> AMEVHPISEFASPFEVFKCIERDFKVAGLLESIGGPQYKARYSVIAWSTNGYLKIHDDPVNILNGYLKDLKLADIPGLFKGGMIGYISYDAVRFWEKIRDLKPAAEDWPYAEFFTPDNIIIYDHNEGKVYVNADLSSVGGCGDIGEFKVSFYDESLNKNSYERIVSESLEYIRSGYIFQVVLSRFYRYIFSGDPLRIYYNLRRINPSPYMFYLKFDEKYLIGSSPELLFRVQDNIVETYPIAGTRPRGADQEEDLKLELELMNSEKDKAEHLMLVDLARNDLGKVCVPGTVKVPELMYVEKYSHVQHIVSKVIGTLKKKYNALNVLSATFPA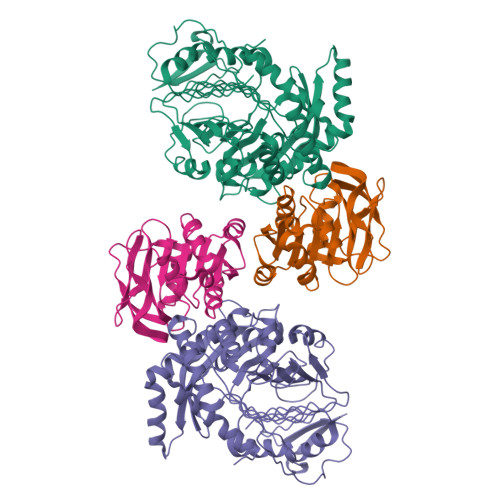GTVSGAPKPMAMNIIETLEEYKRGPYAGAVGFISADGNAEFAIAIRTAFLNKELLRIHAGAGIVYDSNPESEYFETEHKLKALKTAIGVR;> MDLTLIIDNYDSFVYNIAQIVGELGSYPIVIRNDEISIKGIERIDPDRLIISPGPGTPEKREDIGVSLDVIKYLGKRTPILGVCLGHQAIGYAFGAKIRRARKVFHGKISNIILVNNSPLSLYYGIAKEFKATRYHSLVVDEVHRPLIVDAISAEDNEIMAIHHEEYPIYGVQFHPESVGTSLGYKILYNFLNRV(3alpha,8alpha,22R)-cholest-5-ene-3,20,22-triol | C27 H46 O3 | 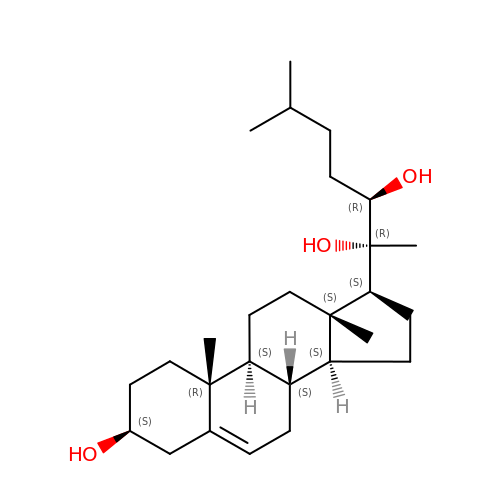ISBSSBGEYIBVTO-TYKWNDPBSA-N> AECKVTVDSTDQM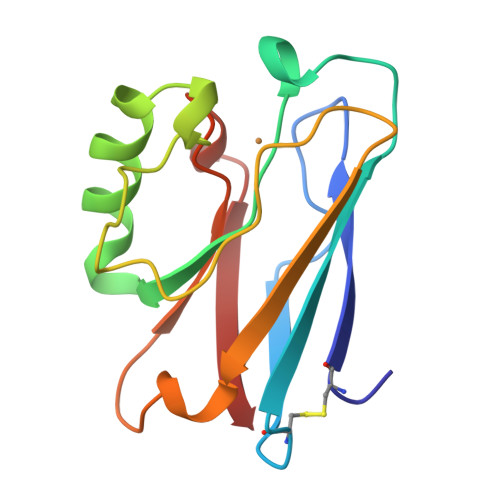SFNTKAIEIDKSCKTFTVELTHSGSLPKNVMGHNWVLSSAADMPGIASDGMAAGIDKNYLKEGDTRVIAHTKIIGAGEKDSVTFDVSKLAAGTDYAFFCSFPGHISMMKGTVTVK> TQVFDLEGYGAISRAMGGTSSSYYTGNAALISNPATLSFAPDGNQFELGLDVVTTDIKVHDSHGAEAKSSTYAVGAQLSYVAQLDDWRFGAGLFVSSGLGTEYGSKSFLSQTENGIQTSFDNSSRLIVLRAPIGFSYQATSKLTFGASVDLVWTSLNLELLLPSSQVGALTAQGNLSGGLVPSLAGFVGTGGAAHFSLSRNSTAGGAVDAVGWGGRLGLTYKLTDNTVLGAMYNFKTSVGDLEGKATLSAISGDGAVLPLDGDIRVKNFEMPASLTLGLAHQFNERWVVAADIKRAYWGDVMDSMNVAFISQLGGIDVALPHRYQDITVASIGTAYKYNNDLTLRAGYSYAQQALDSELILPVIPAYLKRHVTFGGEYDFDKDSRINLAISFGLRERVQTPSYLAGTEMLRQSHSQINAVVSYSKNFHHHHHH

Thus far, only the FadL OM channel family has been shown to mediate transport of hydrophobics. PpF1 has three FadL orthologs, of which TodX (Pput_2883) and CymD (Pput_2901) are located in the adjacent tod and cym/cmt operons respectively. Here we show, by using an integrated approach combining growth assays, X-ray crystallography and molecular dynamics (MD) simulations, that MAH uptake as the first step in biodegradation does occur via lateral diffusion. In the presence of TodX/CymD, robust growth is observed, providing the first direct evidence for MAH transport by FadL-type channels.

We therefore opted to use the same strategy for TodX and CymD, and reasoned that a lack of growth on MAH after closing the lateral opening would provide strong evidence for a lateral diffusion mechanism. The lateral opening in TodX involves both β-strand S2 and S3, contrasting with EcFadL in which only strand S3 is involved. Strand S2 in TodX bulges outward, whereas S3 has a less pronounced kink in the same place as EcFadL. To flatten the S2 bulge, we removed seven residues that were not visible in the density of TodX, replaced a proline with alanine and inserted an alanine to connect the strands (ΔS2). We determined the X-ray crystal structures of both TodX variants which showed that, as expected, the size of the lateral opening is drastically reduced as a result of the flattening of the strands, while the remainder of the mutant structures are very similar to those of wild type. The two TodX mutant channels ΔS2 and ΔS2S3 have much smaller lateral openings, while retaining overall high structural similarity to the wild-type protein. Plate growth assays with vapour-phase toluene showed background growth for the TodX and CymD lateral opening mutants, indicating that they are defective in toluene uptake. For TodX, background growth is already observed for the ΔS2 mutant, so the effect of the additional flattening of strand S3 in the ΔS2S3 variant cannot be assessed.>[2x]MKLTGEVALITGGASGLGRALVDRFVAEGARVAVL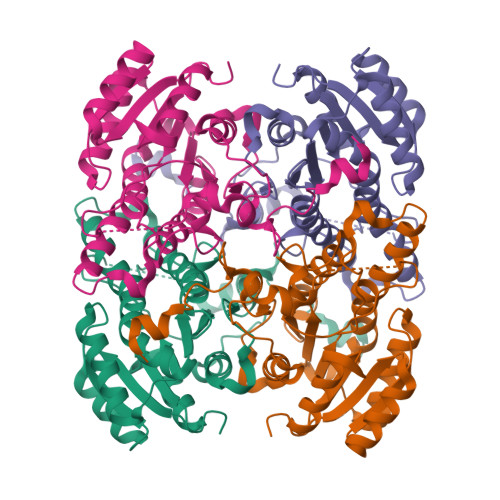DKSAERLRELEVAHGGNAVGVVGDVRSLQDQKRAAERCLAAFGKIDTLIPNAGIWDYSTALADLPEDKIDAAFDDIFHVNVKGYIHAVKACLPALVSSRGSVVFTISNAGFYPNGGGPLYTATKHAVVGLVRQMAFELAPHVRVNGVAPGGMNTDLRGPSSLGLSEQSISSVPLADMLKSVLPIGRMPALEEYTGAYVFFATRGDSLPATGALLNYDGGMGVRGFLTAAGGADLPEKLNINREGQE Type IIS restriction endonucleases (the topic of this study) combine independently folded target recognition (‘TRD’) and endonuclease (‘EN’) domains within a single protein chain, cleaving DNA at one or both sides of their target site. Here, we report biochemical analyses and high-resolution crystallographic and CryoEM structures (in the presence and absence of bound DNA) of the Type IIS REase PaqCI. It forms a tetramer in solution in both the absence and presence of bound DNA, recognizes a longer target than FokI (5′-CACCTGC-3′), and cleaves each strand of bound DNA much closer to the bound target site (4 and 8 bases downstream, respectively). The enzyme displays a similar tetrameric organization of target recognition domains in the absence or presence of bound substrate, with a significant repositioning of endonuclease domains in a trapped DNA-bound complex that is poised to deliver the first of a series of double-strand breaks.

The crystal structure of the DNA-free enzyme was determined to 2.5 Å resolution and found to correspond to a compact enzyme tetramer. In that structure, the asymmetric unit corresponds to an enzyme dimer, with a larger tetrameric assemblage generated via the application of a two-fold crystallographic symmetry axis, forming a dimer-of-dimers. In the crystallographic model, four target recognition domains (TRD) and four endonuclease (EN) domains form a starburst-like structure. The TRDs form a ring of four C-shaped subunits while two EN domains dimerize on either side of the TRD ring, sequestering their active sites against the oligomer and away from solution and DNA. Each dimer pair within the enzyme tetramer contacts the other both through contacts between the sequestered EN domains and through additional contacts between the TRDs. In the unbound structure, the EN domains are held against the TRD ring via contacts between periphery EN loops and a single TRD loop on its neighboring and adjacent monomer. This locks the catalytic domain against the interior of the tetramer and prevents it from cleaving nonspecific DNA duplexes. The resulting data set extended to 2.5 Å resolution and corresponded to a primitive tetragonal space group (P43211) in which two copies of the protein subunit occupied the asymmetric unit. The designation of the enzyme assemblage as a tetramer agrees with (i) the solution behavior of the protein when analyzed and purified via size exclusion chromatography, and (ii) the same structure determined independently via single-particle cryogenic electron microscopy (CryoEM). 3D variability analysis of the CryoEM DNA-free apo-enzyme tetramer map shows an oscillation between either side of the dimer pair, with correlated motions of each TRD affecting the corresponding orientation of its neighbor.

>[2x]MPYDHNAEADFAASEVARMLVADPGLCYDAASLPASISASASYEPSAAGWPKADGLVSVLEGGTSTQRAIALEYKRPQEGIHGLLTAIGQAHGYLHKGYSGAAIVIPGRYSSHPTPAEYVRDVLNAISGSRAIAVFSYSPPDTTSPTPFAGRIQCVRPLVFDAGRVHLRPANQGPKTQWVHMREGSTTRDAFFRFLQVAKRLSADPTAPRPTLRSELVAAIGRLAPGRDPIEYITNTADNKFLTKVWQFFWLEWLATPAVLTPWKLEAGVYSAPGARTRILREDGTDFSQLWEGRVNSLKETIAGMLNRGEISEAQGWEAFVGGISATGGGQDKQGVRARAHSYREDIDSALAQLRWIEDDGLPTDQGYRFMTICERYGGANSRAAIDYMGATLIQTGRYASFLHYINRLSERKFAENPLAYTKPGPGGMPVFTEESYWEYLQDLETKLTDELRVMRKVSGRARPRVRTTFQVELTLLRNYGFVSSTRHRLGVGIPIDWEQVVQALNVDL> MDTEKLMKAGEIAKKVREKAIKLARPGMLLLELAESIEKMIMELGGKPAFPVNLSINEIAAHYTPYKGDTTVLKEGDYLKIDVGVHIDGFIADTAVTVRVGMEEDELMEAAKEALNAAISVARAG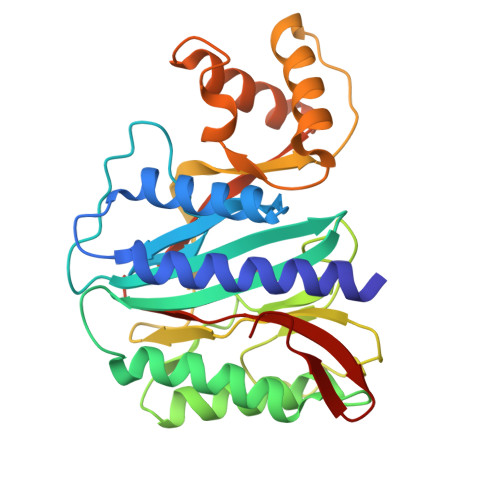VEIKELGKAIENEIRKRGFKPIVNLSGHKIERYKLHAGISIPNIYRPHDNYVLKEGDVFAIEPFATIGAGQVIEVPPTLIYMYVRDVPVRVAQARFLLAKIKREYGTLPFAYRWLQNDMPEGQLKLALKTLEKAGAIYGYPVLKEIRNGIVAQFEHTIIVEKDSVIVTTE>MGKLIRLELFNFKSYKGHHTLLFGDSYFTSIIGPNGSGKSNSMDAISFVLGIKSSHLRSSNLRDLIYRGRVMKTSKIQDDGTTAPATNGDVNGYENGDAGDDEDTSQRTSRNDPKTAWVMAVYEDDAGELHRWKRTITANGTSEYRINDRVVNAQQYNEALEKENILIKARNFLVFQGDVEAIASQSPQDLTRLIEQISGSLEYKEEYERLEEEVRQATEEQAYKLQRRRAANSEIKQYMEQSPGLEVLFMDRLDHVRKQLEQTEQEFEASKAKLRQARESFQAVKQKRLELFNKAFTHIQEQITHVYKELTRSEAYPLGGQAYLDIEEDTDTPFLSGVKYHAMPPLKRFRDMEHLSGGEKTMAALALLFAIHSYQPSPFFVLDEVDAALDNANVEKIKKYIREHAGPGMQFIVISLKPALFQASESLIGVYRDQEANTSRTLTLDLRKYRHH[2x];>[2x]MVTENPQRLTVLRLATNK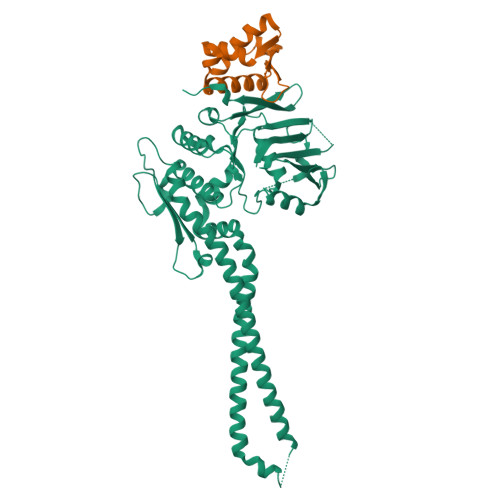GPLAQIWLASNMSNIPRGSVIQTHIAESAKEIAKASGCDDESGDNEYITLRTSGELLQGIVRVYSKQATFLLTDIKDTLTKISMLFKTSQKMTSTVNRLNTVTRVHQLMLEDAVTEREVLVTPGLEFLDDTTIPVGLMAQENSMERKVQGAAPWDTSLEVGRRFSPDEDFEHNNLSSMNLDFDIEEGPITSKSWEEGTRQSSRNFDTHENYIQDDDFPLDDAGTIGWDLGITEKNDQNNDDDDNSVEQGRRLGESIMSEEPTDFGFDLDIEKEAPAGNIDTITDAMTESQPKQTGTRRNSKLLNTKSIQIDEETENSESIASSNTYKEERSNNLLTPQPTNFTTKRLWSEITESMSYLPDPILKNFLSYESLKKRKIHNGREGSIEEPELNVSLNLTDDVISNAGTNDNSFNELTDNMSDFVPIDAGLNEAPFPEENIIDAKTRNEQTTIQTEKVRPTPGEVASKAIVQMAKILRKELSEEKEVIFTDVLKSQANTEPENITKREASRGFFDILSLATEGCIGLSQTEAFGNIKIDAKPALFERFINA>MTTKNTLQPTEAAYIAGFLDGDGSIYAKLIPRPDYKDIKYQVSLAISFIQRKDKFPYLQDIYDQLGKRGNLRKDRGDGIADYTIIGSTHLSIILPDLVPYLRIKK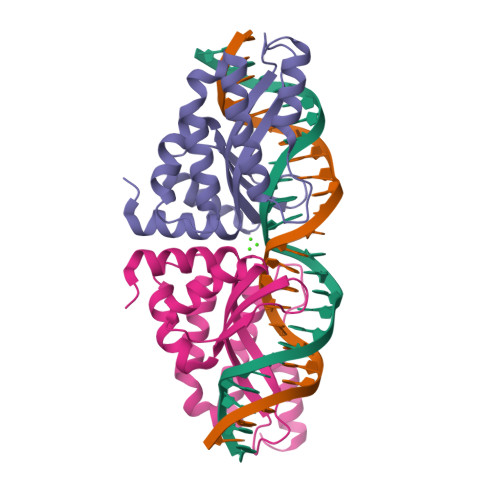KQANRILHIINLYPQAQKNPSKFLDLVKIVDDVQNLNKRADELKSTNYDRLLEEFLKAGKIESSP[2x]> VSAISLPTAPPAAGTESLISGWGNTLSSGADYPDELQCLDAPVLSQA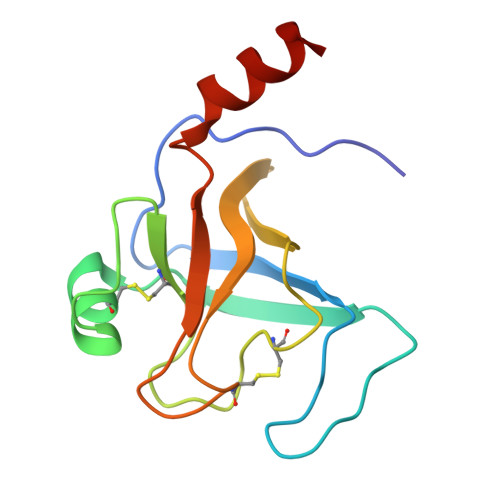ECEASYPGKITNNMFCVGFLEGGKDSCQGDSGGPVVSNGELQGIVSWGYGCAQKNRPGVYTKVYNYVDWIKDTIAANS> MAVDSPDERLQRRIAQLFAEDEQVKAARPLEAVSAAVSAPGMRLAQIAATVMAGYADRPAAGQRAFELNTDDATGRTSLRLLPRFETITYRELWQRVGEVAAAWHHDPENPLRAGDFVALLGFTSIDYATLDLADIHLGAVTVPLQASAAVSQLIAILTETSPRLLASTPEHLDAAVECLLAGTTPERLVVFDYHPEDDDQRAAFESARRRLADAGSLVIVETLDAVRARGRDLPAAPLFVPDTDDDPLALLIYTSGSTGTPKGAMYTNRLAATMWQGNSMLQGNSQRVGINLNYMPMSHIAGRISLFGVLARGGTAYFAAKSDMSTLFEDIGLVRPTEIFFVPRVCDMVFQRYQSELDRRSVAGADLDTLDREVKADLRQNYLGGRFLVAVVGSAPLAAEMKTFMESVLDLPLHDGYGSTEAGASVLLDNQIQRPPVLDYKLVDVPELGYFRTDRPHPRGELLLKAETTIPGYYKRPEVTAEIFDEDGFYKTGDIVAELEHDRLVYVDRRNNVLKLSQGEFVTVAHLEAVFASSPLIRQIFIYGSSERSYLLAVIVPTDDALRGRDTATLKSALAESIQR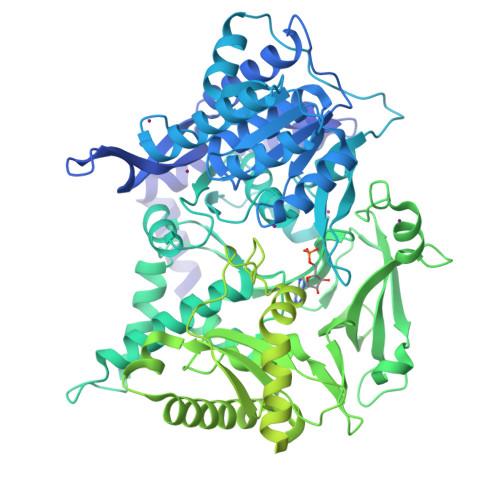IAKDANLQPYEIPRDFLIETEPFTIANGLLSGIAKLLRPNLKERYGAQLEQMYTDLATGQADELLALRREAADLPVLETVSRAAKAMLGVASADMRPDAHFTDLGGDSLSALSFSNLLHEIFGVEVPVGVVVSPANELRDLANYIEAERNSGAKRPTFTSVHGGGSEIRAADLTLDKFIDARTLAAADSIPHAPVPAQTVLLTGANGYLGRFLCLEWLERLDKTGGTLICVVRGSDAAAARKRLDSAFDSGDPGLLEHYQQLAARTLEVLAGDIGDPNLGLDDATWQRLAETVDLIVHPAALVNHVLPYTQLFGPNVVGTAEIVRLAITARRKPVTYLSTVGVADQVDPAEYQEDSDVREMSAVRVVRESYANGYGNSKWAGEVLLREAHDLCGLPVAVFRSDMILAHSRYAGQLNVQDVFTRLILSLVATGIAPYSFYRTDADGNRQRAHYDGLPADFTAAAITALGIQATEGFRTYDVLNPYDDGISLDEFVDWLVESGHPIQRITDYSDWFHRFETAIRALPEKQRQASVLPLLDAYRNPCPAVRGAILPAKEFQAAVQTAKIGPEQDIPHLSAPLIDKYVSDLELLQLL1-(3-methoxyphenyl)methanamine 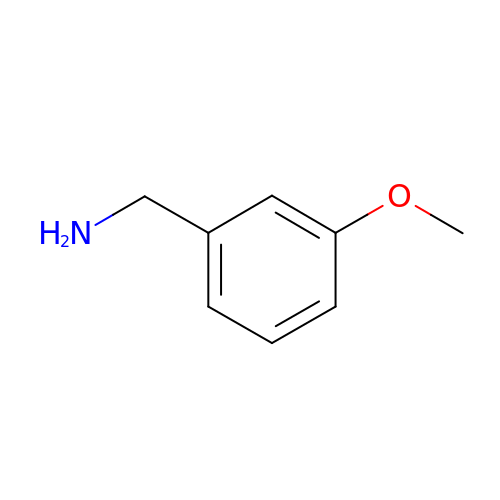| C8 H11 N O | GRRIMVWABNHKBX-UHFFFAOYSA-N>MSLSVAIIGPGAVGTTIAYELQQSLPHTTLIGRHAKTITYYTVPHAPAQDIVVKGYEDVTNTFDVIIIAVKTHQLDAVIPHLTYLAHEDTLIILAQNGYGQLEHIPFKNVCQAVVYISGQKKGDVVTHFRDYQLRIQDNALTRQFRDLVQDSQIDIVLEANIQQAIWYKLLVNLGINSITALGRQTVAIMHNPEIRILCRQLLLDGCRVAQAEGLNFSEQTVDT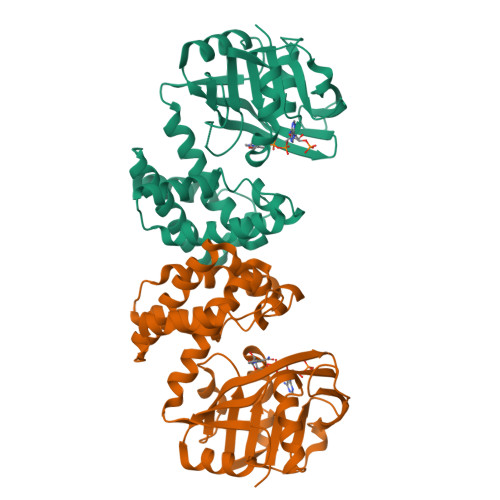IMTIYQGYPDEMGTSMYYDIVHQQPLEVEAIQGFIYRRAREHNLDTPYLDTIYSFLRAYQQNEGHHHHHH[2x]> HHHHHHGSACADPLLPPPPIPAPVSAPATVPPVQNLTALPGGSSNRFSPAPAPAPIASPIPVGAPGSTAVPPLPPPVTPAISGTLRDHLREKGVKLEAQRPHGFKALDITLPMPPRWTQVPDPNVPDAFVVIADRLGNSVYTSNAQLVVYRLIGDFDPAEAITHGYIDSQKLLAWQTTNASMANFDGFPSSIIEGTYRENDMTLNTSRRHVIATSGADKYLVSLSV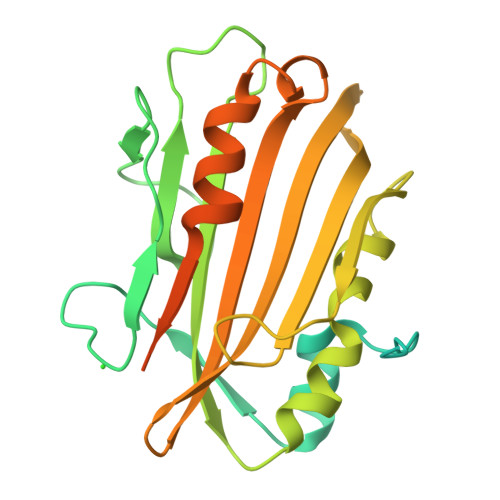TTALSQAVTDGPATDAIVNGFQVVAHAAPAQAPAPAPGSAPVGLPGQAPGYPPAGTLTPVPPR>[2x]TLWRCCQRVVGWVPVLFITFVVVWSYYAYVVELCVFTIFGNEENGKT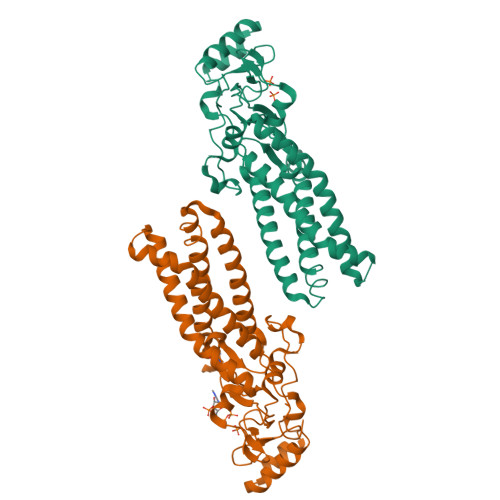VVYLVAFHLFFVMFVWSYWMTIFTSPASPSKEFYLSNSEKERYEKEFSQERQQEILRRAARALPIYTTSASKTIRYCEKCQLIKPDRAHHCSACDSCILKMDHHCPWVNNCVGFSNYKFFLLFLLYSLLYCLFVAATVLEYFIKFWTNELTDTRAKFHVLFLFFVSAMFFISVLSLFSYHCWLVGKNRTTIESFRAPTFSYGPDGNGFSLGCSKNWRQVFGDEKKYWLLPIFSSLGDGCSFPTRLVGM> MEKSKPNVVFVLGGPGSGKGTQCANIVRDFGWVHLSAGDLLRQEQQSGSKDGEMIATMIKNGEIVPSIVTVKLLKNAIDANQGKNFLVDGF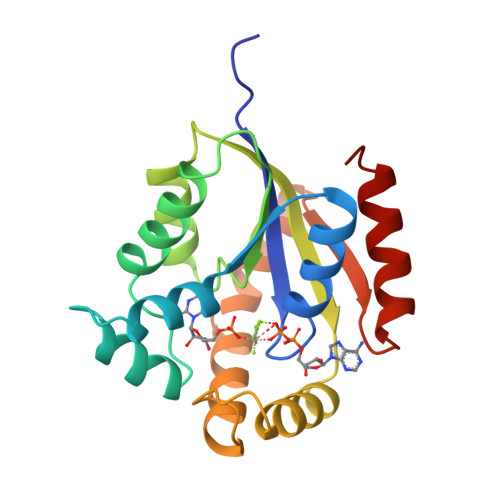PRNEENNNSWEENMKDFVDTKFVLFFDCPEEVMTQRLLKRGESSGRSDDNIESIKKRFNTFNVQTKLVIDHYNKFDKVKIIPANRDVNEVYNDVENLFKSMGF> MLNRISSSSPTSYVSSGSSSAGI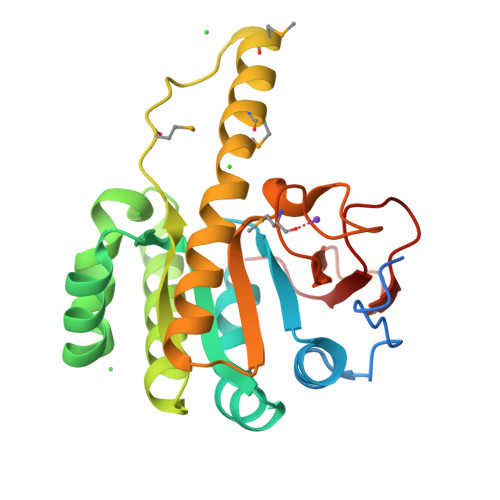NPSINVRPPRGGPVDTLVGAASDNNLVYIGDEHGKLFIPKLITESAAKLKNAGVDHLAVEFVKHSDGAAFREALSDGKSAVKHFLEASWGRHGDAWLDKVSEALCSAHRAGIYVSGIDRKMAIDQPKTPMQKILYMKKRLALNVAWDAAATREASAVCANKSIVWGGAGHFSNSKTDGPKDMRPGLVISFDLTGRGSSRINDADEHSHIVIAGEDN> VVGGLVALRGAHPYIAALYWGHSFCAGSLIAPCWVLTAAHCLQDRPAPEDLTVVLGQERRNHSCEPCQTLAVRSYRLHEAFSPVSYQHDLALLRLQEDADGSCALLSPYVQPVSLPSGAARPSETTLCQVAGWGHQFEGAEEYASFLQEAQVPFLSLERCSAPDVHGSSILPGMLCAGFLEGGTDACQGDSGGPLVCEDQAAERRLTLQGIISWGSGCGDRNKPGVYTDVAYYLAWIREHTVSHHTGTRHHHHH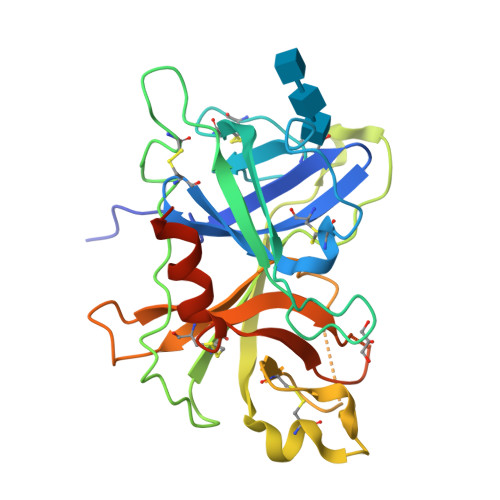H> DYKDDDDLEVLFQGPGGSSAPARPNWLAYDWGLVFLVAAIVALGFVNLGSAAPDPVLLYRQSVALGLGLLLAFLLQFLSRRRLFGLAYPLYGASLLLLALVLVVGREINGARAWFVLGPLQFQPLELAKLGLLLALAKALEGRPIARVWDYALPALLTLPVVGLLLLQPDL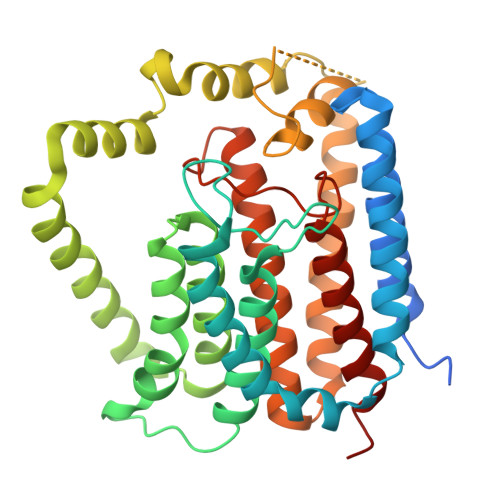GGALVVLFGVFVVVFVRGLPWRHLLVGLFALALLVPTAVWPNLKPYQRERVLIVLDPYRDPLGQGFQVIQSTIAIGSGGLFGKGYGQGTQAQLGFIPFRHTDFVFSVWAEEWGFVGVVGLLGLYGLLLARLFALALACPRLSDRLFLSGFAGMLGFQVVVNLGVALGVMPVTGLTLPLFSYGGSSLIATLAGLGLVLLVHRDRYQD> GPLGSSKVSEQLKCCSGILKEMFAKKHAAYAWPFYKPVDVEALGLHDYCDIIKHPMDMSTIKSKLEAREYRDAQEFGADVRLMFSNCYKYNPPDHEVVAMARKLQDVFEMRFAKMPDEPEEP;> WYDVFLTRK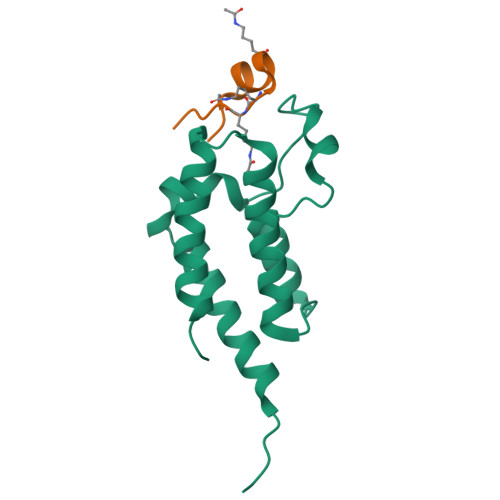YGKKKVAC>DKWEMERTDITMKHKLGGGQYGEVYEGVWKKYSLTVAVKTLKEDTMEVEEFLKEAAVMKEIKHPNLVQLLGVCTREPPFYIITEFMTYGNLLDYLRECNRQEVSAVVLLYMATQISSAMEYLEKKNFIHRDLAARNCLVGENHLVKVADFGLSRLMTGDTFTAHAGAKFPIKWTAPESLAYNKFSIKSDVWAFGVLLWEIATYGMSPYPGIDPSQVYELLEKDYRMERPEGCPEKVYELMRACWQWNPSDRPSFAE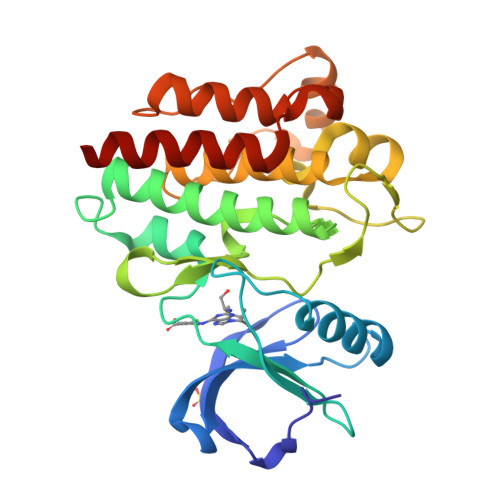IHQAFETMFQESSISD[2x]> AMLPISMSDEGDSFLVKDSLGENKIPKNPSKVVILDLGILDTFDALKLNDKVVGVPAKNLPKYLQQFKNKPSVGGVQQVDFEAINALKPDLIIISGRQSKFYDKLKEIAPTLFVGLDNANFLSSFENNVLSVAKLYGLEKEALEKISDIKNEIEKAKSIVDEDKKALIILTNSNKISAFGPQSRFGIIHDVLGINAVDENIKVGTHGKSINSE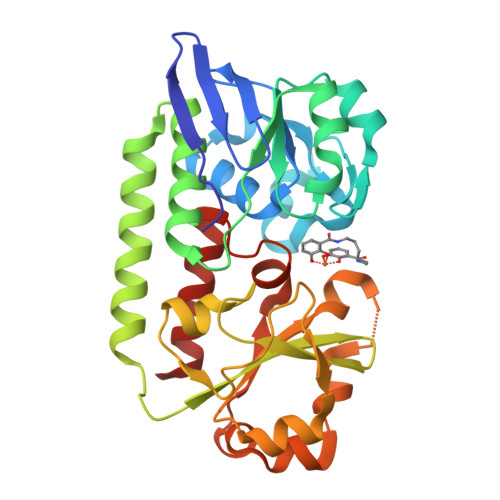FILEKNPDYIFVVDRNVILGNKERAQGILDNALVAKTKAAQNKKIIYLDPEYWYLASGNGLESLKTMILEIKNAVK>APAIQILNFTFDKSVITNGVPSVEFTVTNENDLPVVGLQKMRFAAAQLIPQGATGAGNASQWQYFGDETCDVAATCPGTFVDQKNGHYSYTFNMNLTANAKITYNDQLAQRVLIRAYNTPLPDGTQVPNSNAFVDFTADTGAAPTYSRKIVATESCNTCHQDLANVKHGGAYSDVNYCATCHTAGKVGVGKEFNVLVHAKHKDLTLGSLESCQSCHAANDAAPDWGNWSRIPTAATCGSCHSTVDFAAGKGHSQQLDNSNCIACHNSDWTAELHTGKTADKKAVIAQLGMQATLVGQTDDTAVLTVSILDKDGNAIDAATVQDKIKRLETVTNVGPNFPIMGYNKSPGSGAAKIAKDLVKDGALQAGVTLVDGKLVFTTPALPFGTGDTDTAFTFIGLEMCSTGTSLTACTVDSATTSMKAELAFGTKSGNAPSMRHVNSVNFSTCQGCHSDTFEIHKGHHSGFVMTEQVSHAKDANGKAIVGVDGCVACHTPDGTYASGANKGAFEMKLHVIHGEQGVIKECTQCHNDFNLDAFKVKGALATSAGKYTTPITATCTSCHAPESIGHGLENMGAIVNGDYVQANQAAQSETCFYCHKPTPTDHTQVKM[3x]

Here, we report the atomic structure of an outer membrane spanning protein complex, MtrAB, that is representative of a protein family known to transport electrons between the interior and exterior environments of phylogenetically and metabolically diverse microorganisms. MtrAB is proposed to span the outer membrane and provide electrical connection between the catabolic electron transfer network within the cell, and the electron dispersing MtrC outside the cell (Edwards et al., 2018). Within this complex, the ten heme MtrC is the cell-surface module required when solid-phase minerals serve as terminal electron acceptors (Coursolle and Gralnick, 2010, Hartshorne et al., 2007). The Gram-negative Shewanella is one of the most studied bacterial genera capable of transferring electrons out of the cell to solid-phase Fe(III) and Mn(IV) minerals in order to support anaerobic respiration (Beblawy et al., 2018, Edwards et al., 2018).

To aid initial model building for the Mtr complex, an X-ray crystal structure was obtained for a soluble form of S. baltica OS185 MtrC (MtrCsol). The structure of the monomeric MtrCsol was similar to that of MtrC from S. oneidensis MR-1 described previously (Edwards et al., 2015). MtrCsol consists of 4 domains: two split beta-barrel domains, domains I and III, and two α-helical domains, domains II and IV. These domains serve as a scaffold for 10 bis-His coordinated hemes arranged in a “staggered cross” formation (Edwards et al., 2015). The three MtrCsol monomers within the asymmetric unit of the crystal displayed domain I/II movements relative to domains III/IV. These domain movements centered round a hinge region formed by residues 289–300 located within the alpha helix linking domains II and III. The location of the hinge point suggests this range of motion would not be restricted in the Mtr complex, giving conformational flexibility to MtrC.> RQKDEWAKKTSSLMKQLDWFIGEHLGAMLAAEELG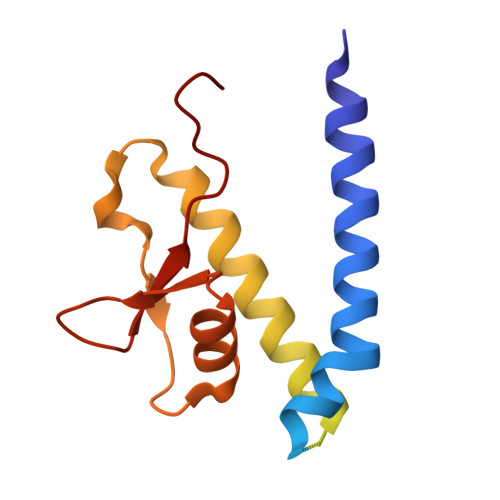GPVVGELMEIDPDDLSAGFNAHGKLKKATSQPDLDRRQRRIDDIWGPQDEQGQAHKRKRGADEALAASAEMRDLIEQLMNKLVEAGGDNSATYVEIPRESAAARFLVRSKVAMFHPNDARRLRLVDFGRDLDD> GSSPSL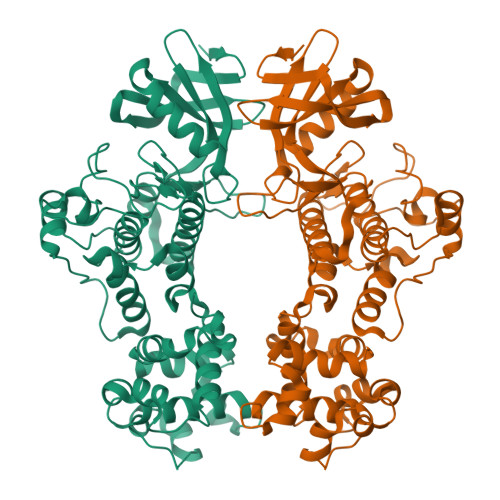EQDDGDEETSVVIVGKISFCPKDVLGHGAEGTIVYRGMFDNRDVAVKRILPECFSFADREVQLLRESDEHPNVIRYFCTEKDRQFQYIAIELCAATLQEYVEQKDFAHLGLEPITLLQQTTSGLAHLHSLNIVHRDLKPHNILISMPNAHGKIKAMISDFGLCKKLAVGRHSFSRRSGVPGTEGWIAPEMLSEDCKENPTYTVDIFSAGCVFYYVISEGSHPFGKSLQRQANILLGACSLDCLHPEKHEDVIARELIEKMIAMDPQKRPSAKHVLKHPFFWSLEKQLQFFQDVSDRIEKESLDGPIVKQLERGGRAVVKMDWRENITVPLQTDLRKFRTYKGGSVRDLLRAMRNKKHHYRELPAEVRETLGSLPDDFVCYFTSRFPHLLAHTYRAMELCSHERLFQPYYFHEPPEPQPPVTPDALGNS>[2x]MGSSHHHHHHSSGLVPRGSHMASAASYPPIKNTKVGLALSSHPLASEIGQKVLEEGGNAIDAAVAIGFALAVVHPAAGNIGGGGFAVIHLANGENVALDFREKAPLKATKNMFLDKQGNVVPKLSEDGYLAAGVPGTVAGMEAMLKKYGTKKLSQLIDPAIKLAENGYAISQRQAETLKEARERFLKYSSSKKYFFKKGHLDYQEGDLFVQKDLAKTLNQIKTLGAKGFYQGQVAELIEKDMKKNGGIITKEDLASYNVKWRKPVVGSYRGYKIISMSPPSSGGTHLIQILNVMENADLSALGYGASKNIHIAAEAMRQAYADRSVYMGDADFVSVPVDKLINKAYAKKIFDTIQPDTVTPSSQIKPGMGQLHEGSN;>ATHYSVADRWGNAVSVTYTINASYGSAASIDGAGFLLNNEMDDFSIKPGNPNLYGLVGGDANAIEANKRPLSSMSPTIVLKNNKVFLVVGSPGGSRIITTVLQVISNV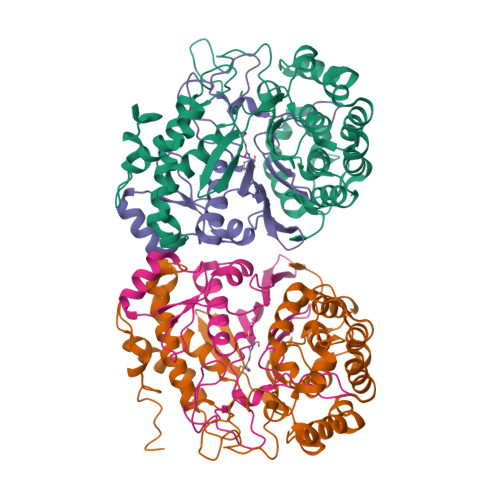IDYNMNISEAVSAPRFHMQWLPDELRIEKFGMPADVKDNLTKMGYQIVTKPVMGDVNAIQVLPKTKGSVFYGSTDPRKEF[2x]UPF3 is a key nonsense-mediated mRNA decay (NMD) factor required for mRNA surveillance and eukaryotic gene expression regulation. UPF3 exists as two paralogs (A and B) which are differentially expressed depending on cell type and developmental stage and believed to regulate NMD activity based on cellular requirements. Here, we show that UPF3A and UPF3B share structural and functional homology to paraspeckle proteins comprising an RNA-recognition motif-like domain (RRM-L), a NONA/paraspeckle-like domain (NOPS-L), and extended α-helical domain. Here, we report two crystal structures of the RRM-L and N-terminal region of the middle-domain of UPF3B and UPF3A bound to the MIF4GIII domain of UPF2.

To study the architecture of UPF3B’s middle-domain we crystallized a construct comprising UPF3B residues 41–189, comprising the RRM-L and the N-terminal part of the middle-domain (NOPS-L), in complex with UPF2-MIF4GIII and solved the structure to 2.6 Å resolution. In good agreement with the predictions from AlphaFold and homology modelling, the beginning of the middle-domain of UPF3B adopts a NOPS-L domain consisting of a linker followed by an α-helix. The area of the structure spanning the RRM-L domain and its interactions with UPF2 align very well with the previously reported UPF3B RRM-L–UPF2-MIF4GIII structure displaying an RMSD of 0.44 Å. The following NOPS-L linker region is composed of conserved residues D148, G152, T153, I154 and D157 which form multiple polar and salt-bridge interactions with R796, K797, L798, and Q794 of helices α1 and α2 of UPF2-MIF4GIII. The subsequent α-helix in the NOPS-L further contributes to UPF2 interaction, primarily through hydrophobic contacts with P770, L771 and Y774 in helices α1 and α2, involving UPF3B residues I154, Y160 and F163. Y167 additionally forms polar contacts with R768 of UPF2-MIF4GIII at the end of the resolvable portion of the helix. Conserved acidic residues D148, D157 and E159 of UPF3B are all interacting with or in close proximity of a basic patch of UPF2-MIF4GIII comprising residues R793, R796, K797 and Q794. Using SPR, we determined a KD between UPF3B-41–189 and UPF2-MIF4GIII of 3.6 nM, which is 200-fold stronger than the KD for the RRM-L alone (720 nM). The contribution of the conserved residues Y160, F163 and Y167, which are buried in a hydrophobic cleft formed by UPF2-MIF4GIII residues P770, L771, Y774, L798 was investigated next. In summary, phosphorylation of UPF3B’s tyrosine residue Y160 or mutation to aspartate results in ∼40-fold reduced UPF2-binding affinity, likely by preventing accommodation of this residue into the hydrophobic cleft formed by UPF2-MIF4GIII.

>[4x]ALSKVVIRRLPPTLTKEQLQEHLQPMPEHDYFEFFSNDTSLYPHMYARAYINFKNQEDIILFRDRFDGYVFLDNKGQEYPAIVEFAPFQKAAKKKTKKRDTKVGTIDDDPEYRKFLESYATD;>[4x]KRPPLQEYVRKLLYKDLSKVTTEKVLRQMRKLPWQDQEVKDYVICCMINIWNVKYNSIHCVANLLAGLVLYQEDVGIHVVDGVLEDIRLGMEVNQPKFNQRRISSAKFLGELYNYRMVESAVIFRTLYSFTSFGVNPDGSPSSLDPPEHLFRIRLVCTILDTCGQYFDRGSSKRKLDCFLVYFQRYVWWKKSLEVWTKDHPFPIDIDYMISDTLELLRPKIKLCNSLEESIRQVQDLEREFLIKLGLVNDK>[2x]MGPVWRKHYITYRINNYTPDMNREDVDYAIRKAFQV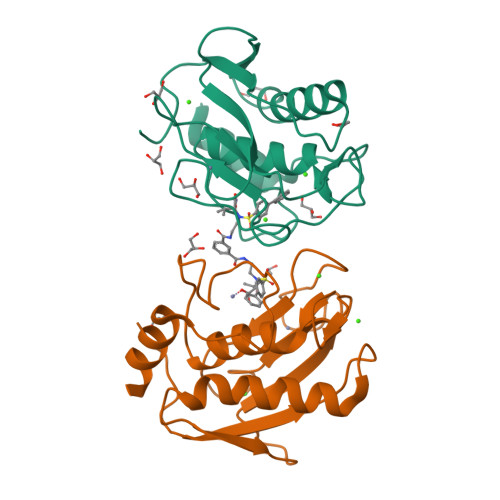WSNVTPLKFSKINTGMADILVVFARGAHGDDHAFDGKGGILAHAFGPGSGIGGDAHFDEDEFWTTHSGGTNLFLTAVHEIGHSLGLGHSSDPKAVMFPTYKYVDINTFRLSADDIRGIQSLYG>[2x]GSHMSKKFALTAEQRASFEKNGFIGPFDAYSPEEMKETWKRTRLRLLDRSAAAYQDLDAISGGTNIANYDRHLDDDFLASHICRPEICDRVESILGPNVLCWRTEFFPKYPGDEGTD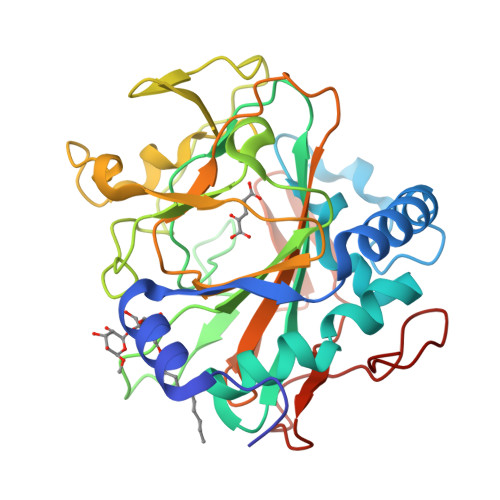WHQADTFANASGKPQIIWPENEEFGGTITVWTAFTDANIANGCLQFIPGTQNSMNYDETKRMTYEPDANNSVVKDGVRRGFFGYDYRQLQIDENWKPDEASAVPMQMKAGQFIIFWSTLMHASYPHSGESQEMRMGFASRYVPSFVHVYPDSDHIEEYGGRISLEKYGAVQVIGDETPEYNRLVTHTTRGKKFEAV2-acetamido-2-deoxy-6-O-phosphono-alpha-D-mannopyranose 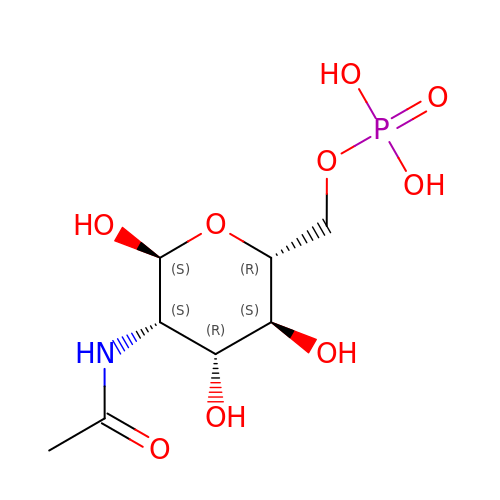| C8 H16 N O9 P | BRGMHAYQAZFZDJ-UOLFYFMNSA-N>[3x]MSSSEDKITVHFINRDGETLTTKGKVGDSLLDVVVENNLDIDGFGACEGTLACSTCHLIFEDHIYEKLDAITDEENDMLDLAYGLTDRSRLGCQICLTKSMDNMTVRVPETVADARQSIDVGKTSAAKKTSSAPRTVLPFEAMPQHPGNRWLRLLQIWREQGYEHLHLEMHQTFQELGPIFRYNLGGPRMVCVMLPEDVEKLQQVDSLHPCRMILEPWVAYRQHRGHKCGVFLLNGPEWRFNRLRLNPDVLSPKAVQRFLPMVDAVARDFSQALKKKVL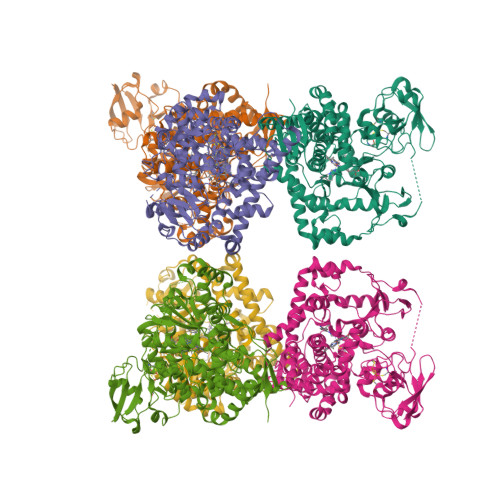QNARGSLTLDVQPSIFHYTIEASNLALFGERLGLVGHSPSSASLNFLHALEVMFKSTVQLMFMPRSLSRWISPKVWKEHFEAWDCIFQYGDNCIQKIYQELAFNRPQHYTGIVAELLLKAELSLEAIKANSMELTAGSVDTTAFPLLMTLFELARNPDVQQILRQESLAAAASISEHPQKATTELPLLRAALKETLRLYPVGLFLERVVSSDLVLQNYHIPAGTLVQVFLYSLGRNAALFPRPERYNPQRWLDIRGSGRNFHHVPFGFGMRQCLGRRLAEAEMLLLLHHVLKHFLVETLTQEDIKMVYSFILRPGTSPLLTFRAINHHHH>[4x]MAVYHMTPPSGWLCNPQRPVTTHGAYQLYYLHSDQNNGPGGWDHASTTDGVAFTHHGTVMPLRPDFPVWSGSAVVDTANTAGFGAGAVVALATQPTDGVRKYQEQYLYWSTDGGFTFTALPDPVIVNTDGRAATTPAEIENAEWFRDPKIHWDTARGEWVCVIGRLRYAAFYT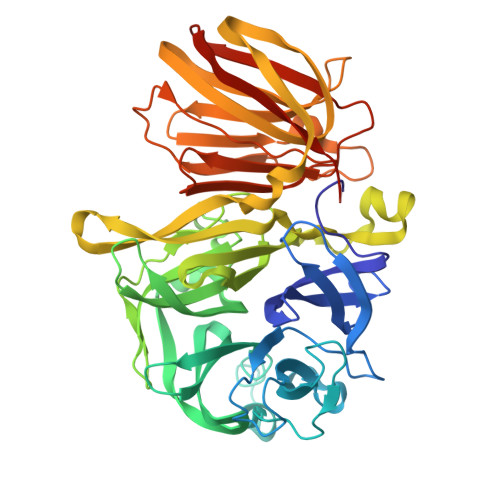SPNLRDWTLRRNFDYPNHALGGIECPDLFEITADDGTRHWVLAASMDAYGIGLPMTYAYWTGTWDGEQFHADDLTPQWLDWGWDWYAAVTWPSIDAPETKRLAIAWMNNWKYAARDVPTDASDGYNGQNSIVRELRLARQPGGWYTLLSTPVAALTNYVTATTTLPDRTVDGSAVLPWNGRAYEIELDIAWDTATNVGISVGRSPDGTRHTNIGKYGADLYVDRGPSDLAGYSLAPYSRAAAPIDPGARSVHLRILVDTQSVEVFVNAGHTVLSQQVHFAEGDTGISLYTDGGPAHFTGIVVREIGQAILEHHHHHHHH>SVSDTNLYSPFKPRNYQLELALPAMKGKNTIICAPTGCGKTFVSLLICEHHLKKFPQGQKGKVVFFANQIPVYEQQKSVFSKYFERHGYRVTGISGATAENVPVEQIVENNDIIILTPQILVNNLKKGTIPSLSIFTLMIFDECHNTSKQHPYNMIMFNYLDQKLGGSSGPLPQVIGLTASVGVGDAKNTDEALDYICKLCASLDASVIATVKHNLEELEQVVYKPQKFFRKVESRISDKFKYIIAQLMRDTESLAKRICKDLENLSQIQNREFGTQKYEQWIVTVQKACMVFQMPDKDEESRICKALFLYTSHLRKYNDALIISEHARMKDALDYLKDFFSNVRAAGFDEIEQDLTQRFEEKLQELESVSRDPSNENPKLEDLCFILQEEYHLNPETITILFVKTRALVDALKNWIEGNPKLSFLKPGILTGRGKTNQNTGMTLPAQKCILDAFKASGDHNILIATSVADEGIDIAQCNLVILYEYVGNVIKMIQTRGRGRARGSKCFLLTSNAGVIEKEQINMYKEKMMNDSILRLQTWDEAVFREKILHIQTHEKFIRDSQEKPKPVPDKENKKLLCRKCKALACYTADVRVIEECHYTVLGDAFKEC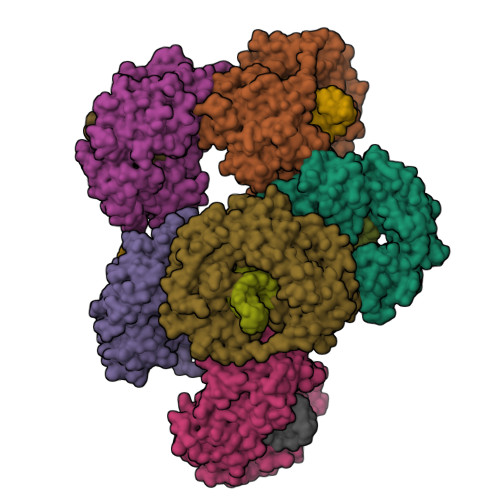FVSRPHPKPKQFSSFEKRAKIFCARQNCSHDWGIHVKYKTFEIPVIKIESFVVEDIATGVQTLYSKWKDFHFEKIPFDPAEMSK[6x]>GSHMVLSNENLNQSLHQEGFSIPLLWLQNCLIRAADDREEDGCSQAVPLVPLTEENEEAMENEQFQQLLRKLGV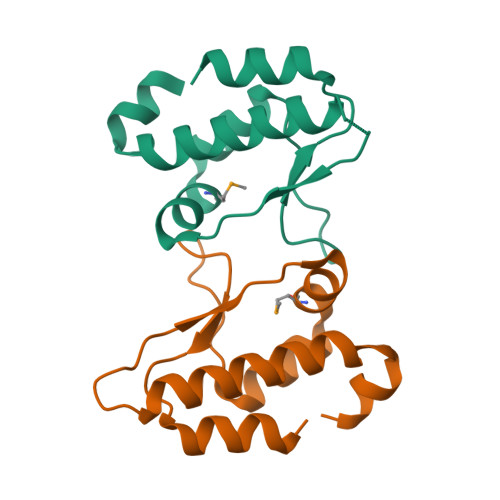RPPASGQETFWRIPAKLSPTQLRRAAASL[4x]AMIDOCARBOXYMETHYLDETHIA COENZYME *A | C23 H39 N8 O17 P3 | 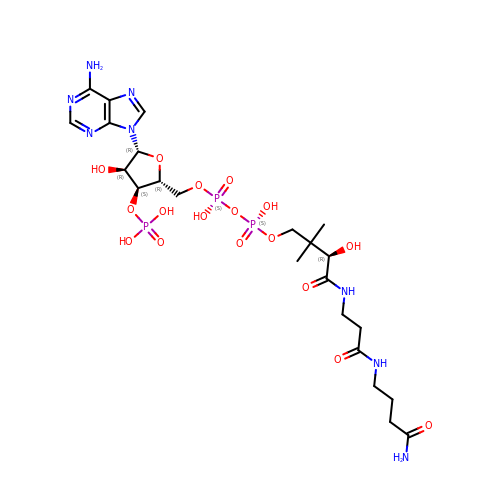RMWCNISNSABOOL-GRFIIANRSA-N>[12x]EDELYRQSLEIISRYLREQATGAKDTKPMGRSGATSRKALETLRRVGDGVQRNHETAFQGMLRKLDIKNEDDVKSLSRVMIHVFSDGVTNWGRIVTLISFGAFVAKH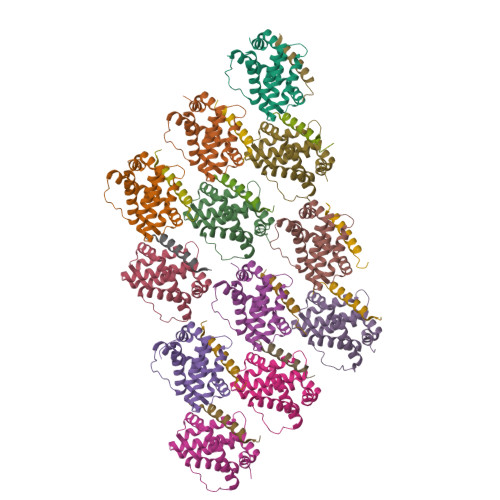LKTINQESCIEPLAESITDVLVRTKRDWLVKQRGWDGFVEFFHVEDLEGG;>PGVMTQEVGQLLQDMGDDVYQQYRSL[12x]High pressure atmospheres of argon and krypton were used to produce noble gas derivatives of crystals of three well studied MPs (two different proton pumps and a sodium light-driven ion pump). The structures obtained using X-ray crystallography showed that the vast majority of argon and krypton binding sites were located on the outer hydrophobic surface of the MPs – a surface usually accommodating hydrophobic chains of annular lipids (which are known structural and functional determinants for MPs). Taken together, the results obtained show that, in addition to binding in internal cavities within the MPs, noble gas atoms interact with MP hydrophobic surface at many sites and displace lipid molecules bound to their surfaces. In the experiments described here, we extend our knowledge as to how noble gas atoms bind to MP molecules, showing that they readily interact with the outer hydrophobic surface of MPs by non-specific binding at multiple sites and in particular compete with binding of lipids to the surfaces of the systems studied.

In total, 47, 35, 11 and 19 noble gas atoms were identified as partially occupying positions in the four crystal structures (tmBR-argon, tmBR-krypton, KR2-krypton, MAR-krypton, respectively). Moreover, at many positions (11, 13, 8 and 6, for tmBR-argon, tmBR-krypton, MAR-krypton and KR2-krypton, respectively), noble gas atoms replaced, at least partially, lipid atoms, with an altered conformation of lipid chains being sometimes clearly visible. Overall, the derivatised structures do not differ significantly from the native ones with Cα r.m.s.d. value not exceeding 0.3 Å; rare side chain position alteration was observed. However, in the particular case of KR2-krypton the backbone of helix E is displaced about 1 Å near the site of two krypton atoms bound in a pocket proximal to ß-ionone ring of the retinal molecule which maintains an unchanged conformation compared to the native crystal structure. In the case of KR2 described here, surface-bound noble gases occupy excavations between α-helices allowing them to closely approach, and perhaps modify, the chemistry of essential co-factors (retinal) by modifying their environment (substantial structural perturbation of the end of helix E). Taking into account the absence of noble gas atoms in central cavities of KR2 molecule, it may be of interest to investigate the functional outcome. Secondly, and most strikingly, all the crystallographically observed positions belonging to the 2nd group (“MP surface” positions) were entirely represented in the results of MD simulations except one krypton position hidden in an excavation, passage to which is blocked by histidine side chain in KR2 structure (in fact, this position is not accessible in the MD experiment as are the internal positions, binding to which requires more significant rearrangements in macromolecule structure).

> MTQELGNANFENFIGATEGFSEIAYQFTSHILTLGYAVMLAGLLYFILTIKNVDKKFQMSNILSAVVMVSAFLLLYAQAQNWTSSFTFNEEVGRYFLDPSGDLFNNGYRYLNWLIDVPMLLFQILFVVSLTTSKFSSVRNQFWFSGAMMIITGYIGQFYEVSNLTAFLVWGAISSAFFFHILWVMKKVINEGKEGISPAGQKILSNIWILFLISWTLYPGAYLMPYLTGVDGFLYSEDGVMARQLVYTIADVSSKVIYGVLLGNLAITLSKNKELVEANS>[2x]MTLVPDLTATDLARHRWLTDNSWTRPTWTVAELEAAKAGRTISVVLPALNEEETVGGVVETIRPLLGGLVDELIVLDSGSTDDTEIRAMAAGARVISREVALPEVAPQPGKGEVLWRSLAATTGDIIVFIDSDLIDPDPMFVPKLVGPLLLSEGVHLVKGFYRRPLKTSGSEDAHGGGRVTELVARPLLAALRPELTCVLQPLGGEYAGTRELLMSVPFAP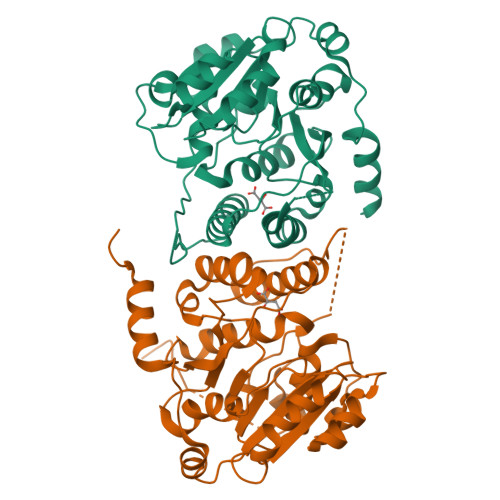GYGVEIGLLVDTYDRLGLDAIAQVNLGVRAHRNRPLTDLAAMSRQVIATLFSRCGVPDSGVGLTQFFADGDGFSPRTSEVSLVDRPPMNTLRGKLAAALEHHHHHH> MQHNAEAAAAAESSTSTVSNLATMATVTASGREVSSGFGPELAADNQDLPDNPTDKSVHNASGASRWSADRGSGPWWLAYEFPGEATISSVNIAWGNTYATNYSIQTSDDGSNWTDVKTGLKATAQAQWVKTTFDTPIKTRHIRMIATTKSQSWSLSVWEMRTMGTISAVATDPLSRLTPRPLYAQSADGEAFELKKNTCVSVSDGSLLPAVDVMRDELGTSYGLKLAEGTNCPITFTLDENLDVTGHVGSAQSITADEAYTIVSDADSVTVKARSATAGIWAAQTLLQL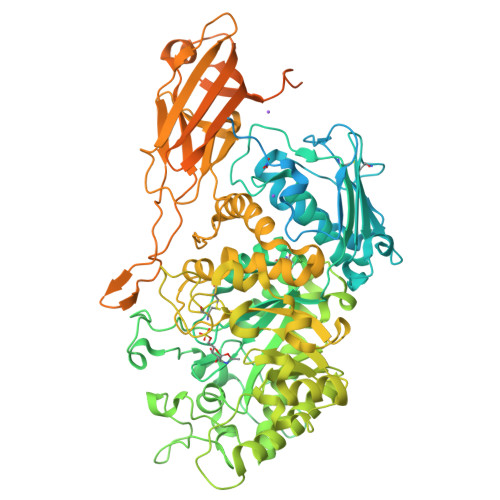IGPWTNSTVKLADVAFIPAVNIADAPRYQWRGVLVDPARSFYPLDEMKQMIDVMSAYKMNTLHLHLSEDEGFRVEITNDGRADGDTTDYTQLAIKSGAISYQSAWTSNWSPAQDGRTGYWTQSEFIELVAYAADHGIAIVPEIDGPGHSFSLLHGLAELNTGNSNPKPAAGEDTPAFIQSAQGRSSLATDADITYTVLGHIMDQLDGMIDKGIKASTMPASELKRMYFHLGGDQLFLSGGAGNKTERLQEYLGRSGALVKERDKTTIVWNDGLDAVDQIPEGSVVQHWTGNAANNASIQKLLNQRNGKIIMSPAGNTYFPQRPGTETTGVTWACGACTTSNFYQWNPTSSAGTTEDKVLGVEDALWSEHLRSLNDAEFLMYTRMMATAEVGWTQQNRKDYDNWNKRVGDIAIDLMNRGANFHKATEVTSWKGSYAAVDAAEQKVTDGKVLVGRYAEPGLTGTDGLSFTATYTAEGGTAVNLPVTPDMKQTYSQQQLKNGRLVVNGAHMNSIVDVYVTLPSDVLAADSEAVGRLDVSVSSSTYPIPSDSSMSIAIKDGKVTQTWTGDERPTPDPDPEPEVTVVSIKASTSQSDVKVGDTFDPSKVKVVATKSDKTTAVLAAADYTIAVTDKDGNAIDVTKPFEAAGDLTVTVALKDDGSIKDSFTMTVTDKGAVDPDPDPTPKPNPDPQKPSGDNKPQIKPEGGKPGDVVAETLEHHHHHH>XGAIQQELKAIQQELKAIQWELKAIQQEL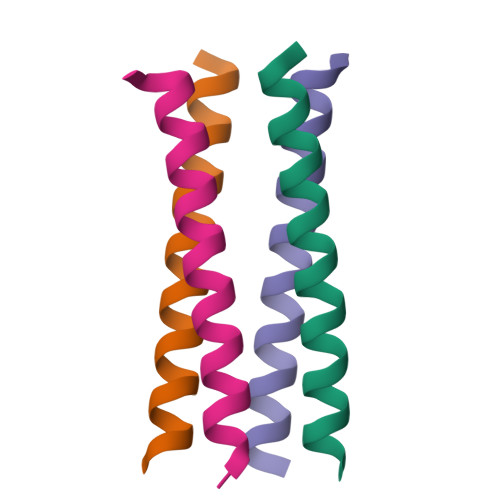KGX[4x]> REFTIDFSTQQSYVSSLNSIRTEISTPLEHISQGTTSVSVINHTPPGSYFAVDIRGLDVYQARFDHLRLIIEQNNLYVAGFVNTATNTFYRFSDFTHISVPGVTTVSMTTDSSYTTLQRVAALERSGMQISRHSLVSSYLALMEFSGNTMTRDASRAVLRFVTVTAEALRFRQIQREFRQALSETAPVYTMT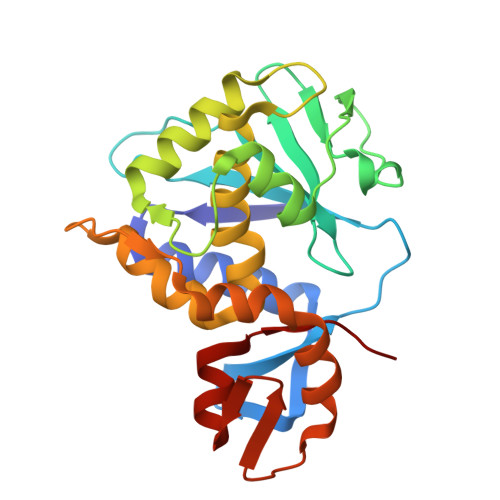PGDVDLTLNWGRISNVLPEYRGEDGVRVGRISFNNISAILGTVAVILNCH>[2x]MAAAAAEEGMEPRALQYEQTLMYGRYTQDLGAFAKEEAARIRLGGPEPWKGPPSSRAAPELLEYGRSRCARCRVCSVRCHKFLVSRVGEDWIFLVLLGLLMALVSWVMDYAIAACLQAQQWMSRGLNTSILLQYLAWVTYPVVLITFSAGFTQILAPQAVGSGIPEMKTILRGVVLKEYLTLKTFIAKVIGLTCALGSGMPLGKEGPFVHIASMCAALLSKFLSLFGGIYENESRNTEMLAAACAVGVGCCFAAPIGGVLFSIEVTSTFFAVRNYWRGFFAATFSAFIFRVLAVWNRDEETITALFKTRFRLDFPFDLQELPAFAVIGIASGFGGALFVYLNRKIVQVMRKQKTINRFLMRKRLLFPALVTLLISTLTFPPGFGQFMAGQLSQKETLVTLFDNRTWVRQGLVEELEPPSTSQAWNPPRANVFLTLVIFILMKFWMSALATTIPVPCGAFMPVFVIGAAFGRLVGESMAAWFPDGIHTDSSTYRIVPGGYAVVGAAALAGAVTHTVSTAVIVFELTGQIAHILPVMIAVILANAVAQSLQPSLYDSIIRIKKLPYLPELGWGRHQQYRVRVEDIMVRDVPHVALSCTFRDLRLALHRTKGRMLALVESPESMILLGSIERSQVVALLGAQLSPARRRQHMQERRATQTSPLSDQEGPPTPEASVCFQVNTEDSAFPAARGETHKPLKPALKRGPSVTRNLGESPTGSAESAGIALRSLFCGSPPPEAASEKLESCEKRKLKRVRISLASDADLEGEMSPEEILEWEEQQLDEPVNFSDCKIDPAPFQLVERTSLHKTHTIFSLLGVDHAYVTSIGRLIGIVTLKELRKAIEGSVTAQGVKVRPPLASFRDSATSSSDTETTEVHALWGPHSRHGLPREGSPSDSDDKCQ

CLC-2 is a voltage-gated chloride channel that contributes to electrical excitability and ion homeostasis in many different tissues. Among the nine mammalian CLC homologs, CLC-2 is uniquely activated by hyperpolarization, rather than depolarization, of the plasma membrane. The TM region of CLC-2 displays a typical CLC family symmetric homodimeric structure, with each subunit containing an independent Cl− pathway. All eukaryotic CLCs contain a pair of ‘cystathionine β-synthase’ (CBS) domains in their intracellular C-terminal domain (CTD).

During the 3D classification data processing with a C1 reconstruction (no symmetry imposed), two distinct conformations were separated from the same CLC-2 dataset. The main structural differences occur at the intracellular domain, with one class exhibiting a symmetric arrangement and the other, asymmetric. These two conformations are named as CLC2-CTDsym and CLC2-CTDasym, respectively (Figure 4—figure supplements 1 and 2). In the asymmetric arrangement (CLC2-CTDasym), one of the CTDs rotates toward the TM region approximately 35° relative to the conformation in the symmetric structure. Structural comparison focused on individual CTDs within the two classes reveals low RMSD values (~1 Å), which indicates that the CTD undergoes a rigid body movement to accomplish the conformational change. In CLC2-CTDasym, only the subunit whose CTD adopts the ‘symmetric’ orientation (seen in CLC2-CTDsym) contains the hairpin density; in the subunit with the rotated CTD, no hairpin density is observed. Along with the absence of hairpin density, the subunit with the rotated CTD exhibits a difference in the linker connecting TM helices J and K, which is poorly resolved and insufficient for model building. A key aspect of our revised framework is that ball-and-chain gating is coupled to CTD conformational change: close examination of the state with the CTD rotated reveals that the hairpin cannot access its pore-blocking site in this state. Thus, CTD rotation facilitates hairpin release and channel opening. In contrast to CLC-0, where movements in the CTD have been linked to the highly cooperative conformational change involved in common gating, our structures illustrate that in CLC-2 the CTDs can move independently of one another.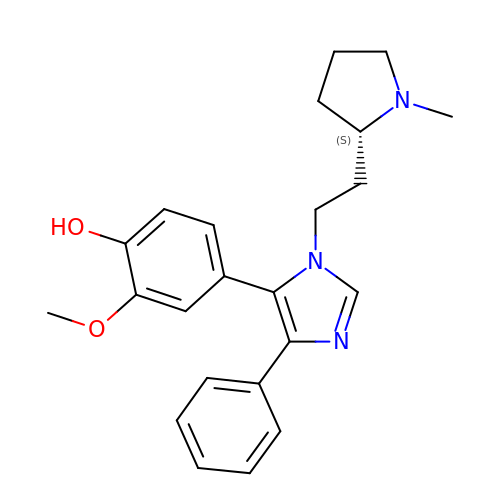2-methoxy-4-(1-{2-[(2S)-1-methylpyrrolidin-2-yl]ethyl}-4-phenyl-1H-imidazol-5-yl)phenol | C23 H27 N3 O2 | YGPHAIXUDLLWHC-IBGZPJMESA-N>[4x]MATVHKVGDSTGWTTLVPYDYAKWASSNKFHVGDSLLFNY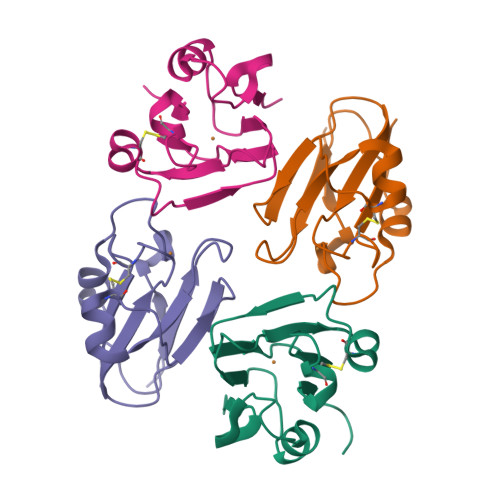NNKFHNVLQVDQEQFKSCNSSSPAASYTSGADSIPLKRPGTFYFLCGIPGHCQLGQKVEIKVDPGSSSA The genomes of most C. perfringens strains contain three separate genes encoding highly conserved GH33 CAZymes targeting sialic acid glycosidic linkages: the nonsecreted 43 kDa NanH, and the two secreted 77 kDa NanI and 129 kDa NanJ. Here, we present the structural and biochemical characterization of the GH33 catalytic domains of the three sialidases of C. perfringens and probe their substrate specificity. The catalytically active domains, which we refer to as NanHGH33, NanJGH33, and NanIGH33, displayed differential activity on various naturally occurring forms of sialic acid. We report the X-ray crystal structures of these domains in complex with relevant sialic acid variants revealing the molecular basis of how each catalytic domain accommodates different sialic acids.

NanJ is highly multimodular comprising a central GH33 domain flanked on the N terminus by family 32 and 40 CBMs and on the C-terminal side by an unknown domain, X82 cohesin, and fibronectin type III-like domains. The structures of NanHGH33 and NanJGH33 display the characteristic 6-bladed β-propeller fold seen in exo-acting sialidase GH33 domains. The structures of NanJGH33 and NanIGH33 were very similar with an RMSD of 1.1 Å and with both proteins containing the same β-sheet domain insertion within the catalytic domain (between residues 477–546 in NanJGH33 and 361–427 in NanIGH33). The inserted domain is not present in NanHGH33 and the RMSD of NanHGH33 with the other two structures is 1.7 Å. The inserted domain is not within the proximity of the catalytic site of the sialidases, and therefore likely does not directly impact the activity of the sialidase. The amino acid side chains forming the active site pockets of NanJGH33 and NanIGH33 were identical, though a notable position in a second shell of active site residues showed a tryptophan (W354 in NanIGH33) versus proline (P472 in NanJGH33) difference. In contrast, these loops are relatively minimal in NanIGH33 and NanJGH33, creating a somewhat shallow sialic acid binding site. This lack of a +1 binding site in either NanIGH33 or NanJGH33 supports a general absence of selectivity for α-2,3- or α-2,6- linkages. However, NanI is predicted to be fully secreted while NanJ has a cohesin module that participates in the formation of CAZyme complexes and an FN3 domain that is postulated to mediate attachment to the bacterial cell-surface.

> MDDVYKTQPVELFYPGYLESRGYRIPALETTKKGTVLASIDVRNNGDHDAPNNNIDVGIRRKEVNGEWEEGKVILDYPGKSAAIDTSLMSATIEENGIEKERIFLIVTHFPEGYGFPNTEGGSGYKEIDGKYYFILKDAQNNEYTVREDGIVYNSEGNETDYVMKNDKTLIQNGEEVGNALLSNSPLKAVGTAHIEMIYSDDDGNTWSEPEDLNPGLKKEWMKFFGTAPGKGIQIKNGEHKGRLVFPIYYTNQNNFQSSAVIYSDDFGETWKLGESPIDTASVSSETVSSGTQLTECQVVEMPNGQLKLFMRNTGSYTRIATSFDGGATWHDEVPEDTSLREPYCQLSVINYSGKINGKDAIIFSNPDASSRVNGSVKVGLINENGTYDNGEPRYEFDWIYNKTVKPGSFAYSCLTELPDGNLGLFYEGEGAGRMAYTEFDLNYLKFNA> GMHTDVNALFAALWQDYIKMTPSAAKIHQLLGHGAPIINDHIALRTFNIAKVNLSVLAKHFTSIGYVDS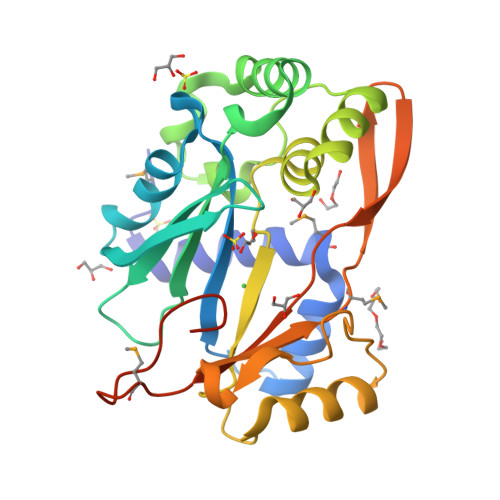GDYKFEQKKLIAKHFEHPDPKQPKVFISELLVEEFSPEVQKSIHGLIDQVDIAATTADNFIYSGRHWDVDKATYQALLAESEYAAWVAALGYRANHFTVSINDLPEFERIEDVNQALKQAGFVLNSSGGEVKGSPEVLLEQSSTMADKVVVNFTDGDVEIPSCFYEFARRYPMANGQLYTGFVAASADKIFESTNAMM> CUGGGUC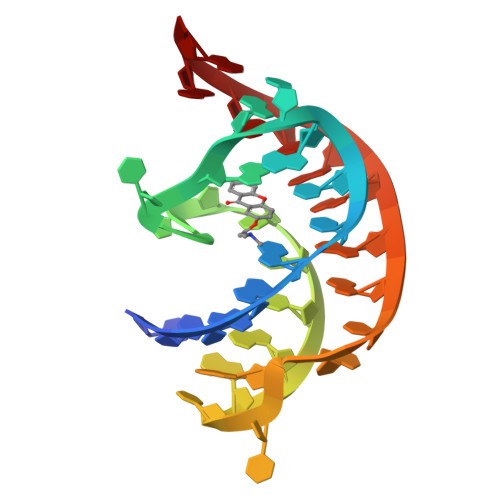GCAGUNNNCCCAGUUAACAAAACAAG> MGLIEKIVDWIDERAHVREIYRTQMVEYKVAKNLTFPYVFGILALVTFAIQIISGMVLILYYKPSIADAFDSATYSIMGEIPFGWLFRHIHATGANFFMAIVYLHMFTGIYYNAYKRPRELVWIVGWLIYFVLILTALSGYLLPWGQLSYWGFIVTTEIPGSLADAPILKPIFKAIAETIVLWMKGGYVVTDVTLGRVFGSHVLIYPLILLALVGIHLYLVRAAGISNPEGIEYDKKKNPDKFVPFHPYMTLKEGAYVMWYLAVFFFFVFFHISHFLPPENFEPANPLKTPAHIAPEWYLLGYYEVFRSIPSKFWGFVAFNALLLLLLLLPFLDFSPLKSARRRPLFFVMFVIFMI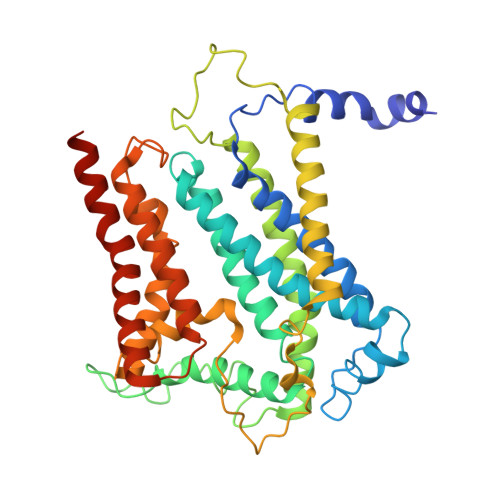SSMALTILGTMPPTPQNAKLGLIFAALVFAFFISLPIISFIEYGWYKAKGGQQE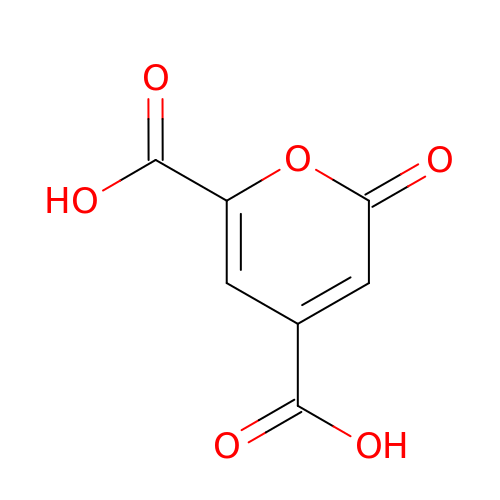2-oxo-2H-pyran-4,6-dicarboxylic acid | C7 H4 O6 | VRMXCPVFSJVVCA-UHFFFAOYSA-N> GSNHHRGLASANVDFAFSLYKHLVALSPKKNIFISPVSISMALAMLSLGTCGHTRAQLLQGLGFNLTERSETEIHQGFQHLHQLFAKSDTSLEMTMG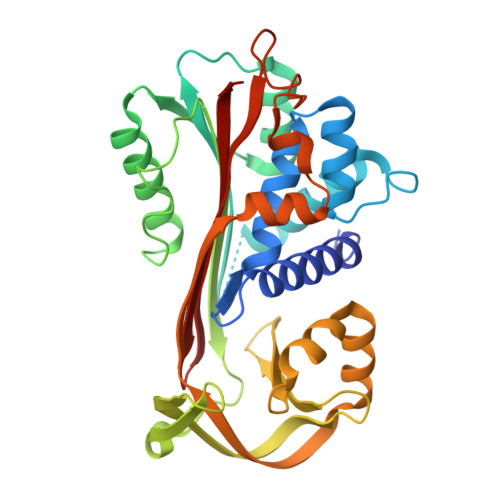NALFLDGSLELLESFSADIAHYYESEVLAMNFQDWATASRQINSYVKNKTQGKIVDLFSGLDSPAILVLVNYIFFKGTWTQPFDLASTREENFYVDETTVVKVPMMLQSSTISYLHDSELPCQLVQMNYVGNGTVFFILPDKGKMNTVIAALSRDTINRWSAGLTSSQVDLYIPKVTISGVYDLGDVLEEMGIADLFTNQANFSRITQDAQLKSSKVVHKAVLQLNEEGVDTAGSTGVTLNLT>MGDEDKRITYEDSEPSTGMNYTPSMHQEAQEETVMKLKGIDANEPTEGSILLKSSEKKLQETPTEANHVQRLRQMLACPPHGLLDRVITNVTIIVLLWAVVWSITGSECLPGGNLFGIIILFYCA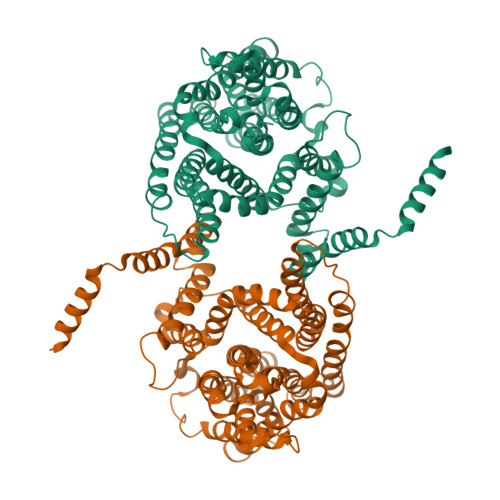IIGGKLLGLIKLPTLPPLPSLLGMLLAGFLIRNIPVINDNVQIKHKWSSSLRSIALSIILVRAGLGLDSKALKKLKGVCVRLSMGPCIVEACTSALLAHYLLGLPWQWGFILGFVLGAVSPAVVVPSMLLLQGGGYGVEKGVPTLLMAAGSFDDILAITGFNTCLGIAFSTGSTVFNVLRGVLEVVIGVATGSVLGFFIQYFPSRDQDKLVCKRTFLVLGLSVLAVFSSVHFGFPGSGGLCTLVMAFLAGMGWTSEKAEVEKIIAVAWDIFQPLLFGLIGAEVSIASLRPETVGLCVATVGIAVLIRILTTFLMVCFAGFNLKEKIFISFAWLPKATVQAAIGSVALDTARSHGEKQLEDYGMDVLTVAFLSILITAPIGSLLIGLLGPRLLQKVEHQNKDEEVQGETSVQV[2x]>AAGAAPVDISTLPRVKVDLVKPPFVHAHDQVAKTGPRVVEFTMTIEEKKLVIDREGTEIHAMTFNGSVPGPLMVVHENDYVELRLIN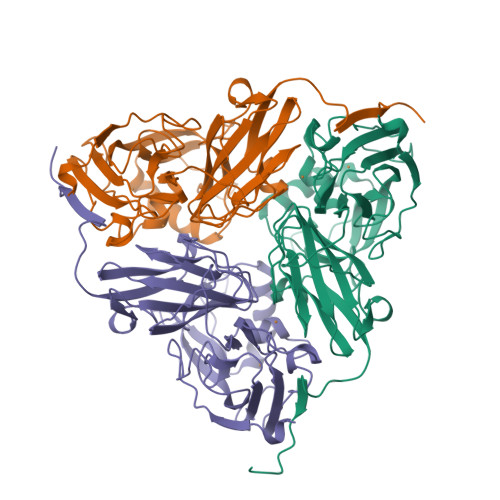PDTNTLLHNIDFHAATGALGGGALTQVNPGEETTLRFKATKPGVFVYHCAPEGMVPWHVTSGMNGAIMVLPRDGLKDEKGQPLTYDKIYYVGEQDFYVPKDEAGNYKKYETPGEAYEDAVKAMRTLTPTHIVFNGAVGALTGDHALTAAVGERVLVVHSQANRDTRPHLIGGHGDYVWATGKFRNPPDLDQETWLIPGGTAGAAFYTFRQPGVYAYVNHNLIEAFELGAAGHFKVTGEWNDDLMTSVVKPASM[3x]> MGPGAPFARVGWPLPLLVVMAAGVA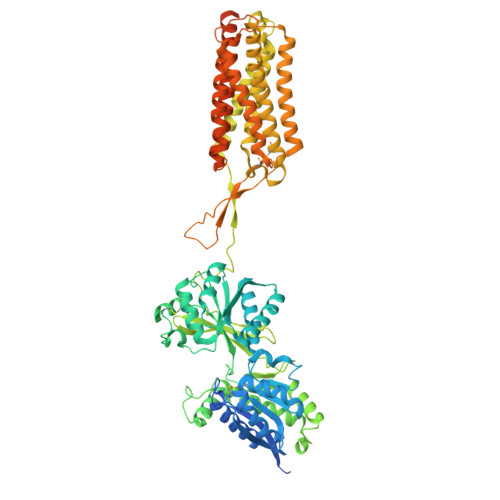PVWASHSPHLPRPHSRVPPHPSSERRAVYIGALFPMSGGWPGGQACQPAVEMALEDVNSRRDILPDYELKLIHHDSKCDPGQATKYLYELLYNDPIKIILMPGCSSVSTLVAEAARMWNLIVLSYGSSSPALSNRQRFPTFFRTHPSATLHNPTRVKLFEKWGWKKIATIQQTTEVFTSTLDDLEERVKEAGIEITFRQSFFSDPAVPVKNLKRQDARIIVGLFYETEARKVFCEVYKERLFGKKYVWFLIGWYADNWFKIYDPSINCTVDEMTEAVEGHITTEIVMLNPANTRSISNMTSQEFVEKLTKRLKRHPEETGGFQEAPLAYDAIWALALALNKTSGGGGRSGVRLEDFNYNNQTITDQIYRAMNSSSFEGVSGHVVFDASGSRMAWTLIEQLQGGSYKKIGYYDSTKDDLSWSKTDKWIGGSPPADQTLVIKTFRFLSQKLFISVSVLSSLGIVLAVVCLSFNIYNSHVRYIQNSQPNLNNLTAVGCSLALAAVFPLGLDGYHIGRNQFPFVCQARLWLLGLGFSLGYGSMFTKIWWVHTVFTKKEEKKEWRKTLEPWKLYATVGLLVGMDVLTLAIWQIVDPLHRTIETFAKEEPKEDIDVSILPQLEHCSSRKMNTWLGIFYGYKGLLLLLGIFLAYETKSVSTEKINDHRAVGMAIYNVAVLCLITAPVTMILSSQQDAAFAFASLAIVFSSYITLVVLFVPKMRRLITRGEWQSEAQDTMKTGSSTNNNEEEKSRLLEKENRELEKIIAEKEERVSELRHQLQSRDYKDDDDK> MGSMLFFSFFKTLVDQEVVVELKNDIEIKGTLQSVDQFLNLKLDNISCTDEKKYPHLGSVRNIFIRGSTVRYV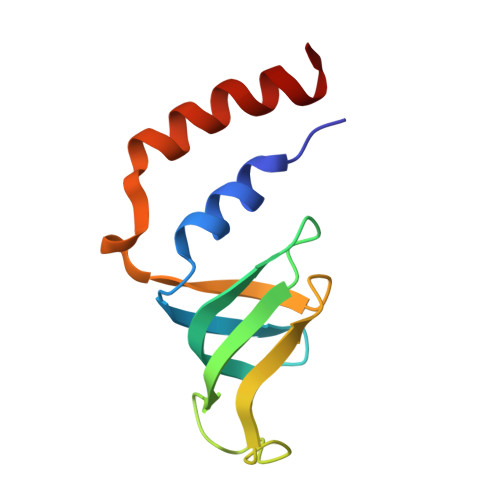YLNKNMVDTNLLQDATRREVMTERK>[2x]MQVKPCTPEFYQTHFQLAYRLQSRPRGLALVLSNVHFTGEKELEFRSGGDVDHSTLVTLFKLLGYDVHVLCDQTAQEMQEKLQNFAQLPAHRVTDSCIVALLSHGVEGAIYGVDGKLLQLQEVFQLFDNANCPSLQNKPKMF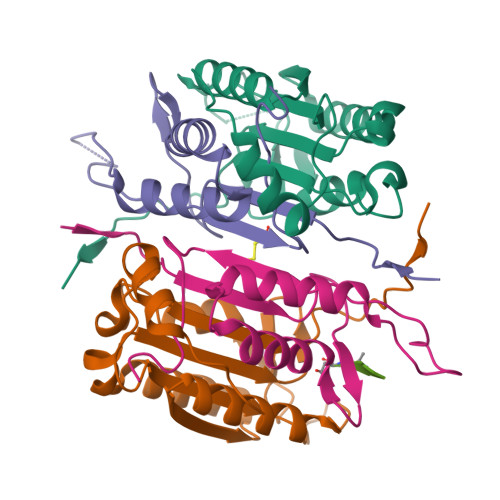FIQACRGDETDRGVDQQD;>[2x]GKEKLPKMRLPTRSDMICGYACLKGTAAMRNTKRGSWYIEALAQVFSERACDMHVADMLVKVNALIKDREGYAPGTEFHRCKEMSEYCSTLCRHLYLFPGHPPTLEHHHHHH;> XDVAD>[4x]MGSSHHHHHHSSGLVPRGSTSYGIQKGNQPEGSMVFTVSRDSLPGYESFGT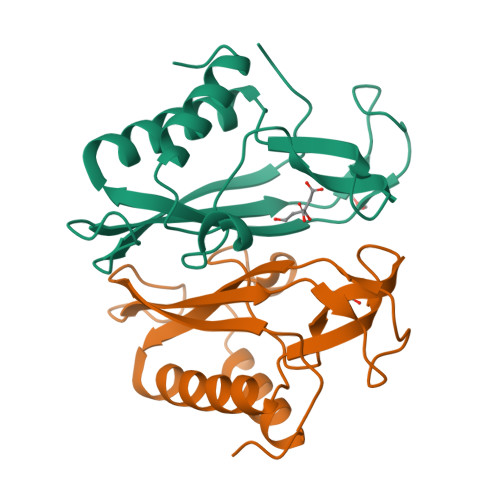IVITYSMKAGIQTEEHPNPGKRYPGIQRTAYLPDNKEGRKVLKLLYRAFDQKLIFTVGYSRVLGVSDVITWNDIHHKTSRFGGPEMYGYPDPSYLKRVKEELKAKGIE~{N}-methyl-~{N}-octyl-3,4,5-tris(oxidanyl)benzamide | C16 H25 N O4 | 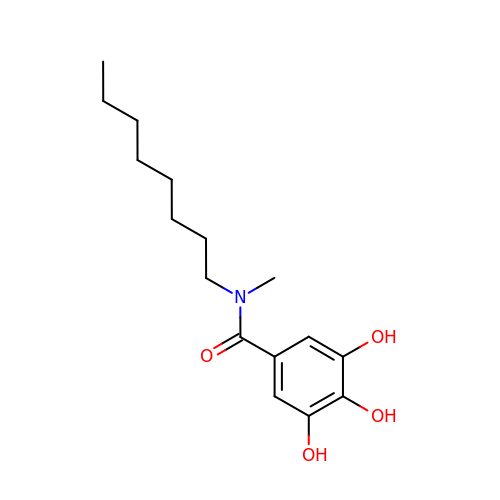HUVVKGRTMBOPNF-UHFFFAOYSA-N>MLKQVEIFTDGSCLGNPGPGGYGAILRYRGREKTFSAGYTRTTNNRMELMAAIVALEALKEHCEVILSTDSQYVRQGITQWIHNWKKRGWKTADKKPVKNVDLWQRLDAALGQ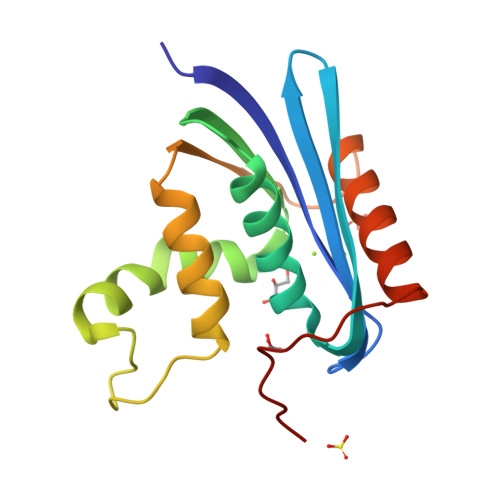HQIKWEWVKGHAGHPENERCDELARAAAMNPTLEDTGYQVEV[2x]(2~{S})-2-azanyl-3-(1~{H}-indol-3-yl)-~{N}-[2-(2,4,6-trimethylphenyl)ethyl]propanamide | C22 H27 N3 O | 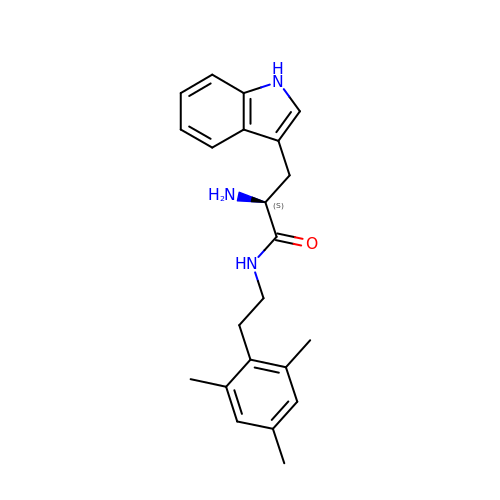BQKLGIPTHQLBPK-FQEVSTJZSA-N> MGSSHHHHHHSSGLVPRGSMKSNSKDSENKKVENLVLDDNDENTIIPYYLSNLLTNPSNPVVFMDINLGNNFLGKFKFELFQNIVPKTSENFRQFCTGEYKVNNLPVGYKNTIFHRVIKEFMIQGGDFINHNGSGSLSIYGEKFDDENFDIKHDKEGLLSMANSGPNTNGCQFFITTKKCEWLDGKNVVFGRIIDNDSLLLLKKIENVSVTPYI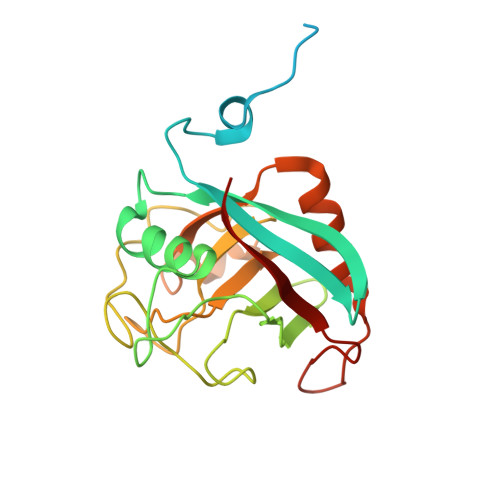YKPKIPINVVECGEL>GSHMTELLKNHVAGQWIAGTGAGITLTDPVTGVALVRVSSEGLDLARAFSFAREDGGAALRALTYAQRAARLADIVKLLQAKRGDYYAIATANSGTTRNDSAVDIDGGIFTLSYYAKLGASLGEVHALRDGSAESLSKDRSFSAQHVLSPTRGVALFINAFNFPSWGLWEKAAPALLSGVPVIVKPATATAWLTQ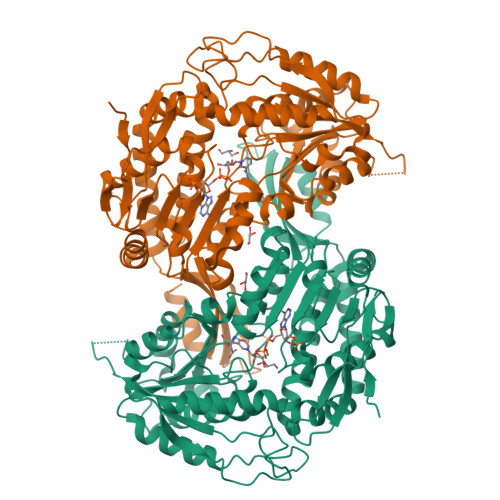RMVADVVDAGILPPGALSIICGSSAGLLDQIRSFDVVSFTGSADTAATLRAHPAFVQRGARLNVQADSLNSAILCADATPDTPAFDLFIKEVVREMTVKSGQKCTAIRRAFVPEAALEPVLEALKAKLAKITVGNPRNDAVRMGSLVSREQYENVLAGIAALREEAVLAYDSSAVPLIDADANIAACVAPHLFVVNDPDNATLLHDVEVFGPVASVAPYRVTTDTNALPEAHAVALARRGQGSLVASIYSNDDAHLGRLALELADSHGRVHAISPSVQHSQTGHGNVMPMSLHGGPGRAGGGEELGGLRALAFYHRRSAIQAASAAIGTLTQATHWPAA[2x]>KGKLPPVYPVTVPILGHIIQFGKSPLGFMQECKRQLKSGIFTINIVGKRVTIVGDPHEHSRFFLPRNEVLSPREVYSFMVPVFGEGVAYAAPYPRMREQLNFLAEELTIAKFQNFVPAIQHEVRKFMAANWDKDEGEINLLEDCSTMIINTACQCLFGEDLRKRLDARRFAQLLAKMESSLIPAAVFLPILLKLPLPQSARCHEARTELQKILSEIIIARKEEEVNKDSSTSDLLSGLLSAVYRDGTPMSLHEVCGMIVAAMFAGQHTSSITTTWSMLHLMHPANVKHLEALRKEIEEFPAQLNYNNVMDEMPFAERCARESIRRDPPLLMLMRKVMADVKVGSYVVPKGDIIACSPLLSHHDEEAFPEPRRWDPERDEKVEGAFIGFGAGVHKCIG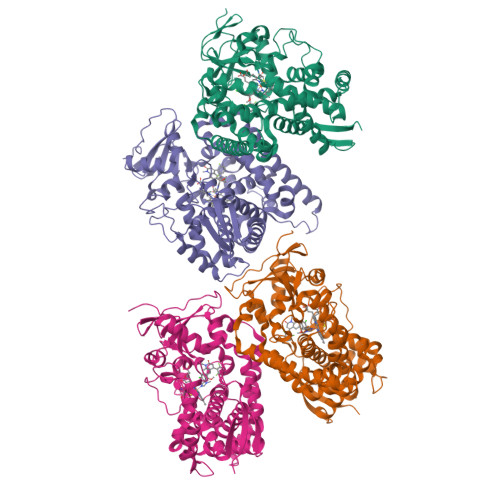QKFGLLQVKTILATAFRSYDFQLLRDEVPDPDYHTMVVGPTASQCRVKYIRRKAAAA[4x]> GLGQMLESMIDNTVRETVGAATSRDALPNTEASGPTHSKEIPALTAVETGATNPLVPSDTVQTRHVVQHRSRSESSIESFFARGACVTIMTVDNPASTTNKDKLFAVWKITYKDTVQLRRKLEFFTYSRFDMELTFVVTANFTETNNGHALNQVYQIMYVPPGAPVPEKWDDYTWQTSSNPSIFYTYGTAPARISVPYVGISNAYSHFYDGFSKVPLKDQSAALGDSLYGAASLNDFGILAVRVVNDHNPTKVTSKIRVYLKPKHIRVWCPRPPRAVAYYGPGVDYKDGTLTPLSTKDLTTY;> SPNIEACGYSDRVLQLTLGNSTITTQEAANSVVAYGRWPEYLRDSEANPVDQPTEPDVAACRFYTLDTVSWTKESRGWWWKLPDALRDMGLFGQNMYYHYLGRSGYTVHVQCNASKFHQGALGVFAVPEMCLAGDSNTTTMHTSYQNANPGEKGGTFTGTFTPDNNQTSPARRFCPVDYLLGNGTLLGNAFVFPHQIINLRTNNCATLVLPYVNSLSIDSMVKHNNWGIAILPLAPLNFASESSPEIPITLTIAPMCCEFNGLRNITLPRLQ;> GLPVMNTPGSNQYLTADNFQSPCALPEFDVTPPIDIPGEVKNMMELAEIDTMIPFDLSATKKNTMEMYRVRLSDKPHTDDPILCLSLSPASDPRLSHTMLGEILNYYTHWAGSLKFTFLFCGSMMATGKLLVSYAPPGADPPKKRKEAMLGTHVIWDIGLQSSCTMVVPWISNTTYRQTIDDSFTEGGYISVFYQTRIVVPLSTPREMDILGFVSACNDFSVRLLRDTTHIEQKALAQ;> XGAQVSSQKVGAHENSNRAYGGSTINYTTINYYRDSASNAASKQDFSQDPSKFTEPIKDVLIKTAPMLN;> MARAMAAAWPLLLVALLVLSWPPPGTGDVVVQAPTQVPGFLGDSVTLPCYLQVPNMEVTHVSQLTWARHGESGSMAVFHQTQGP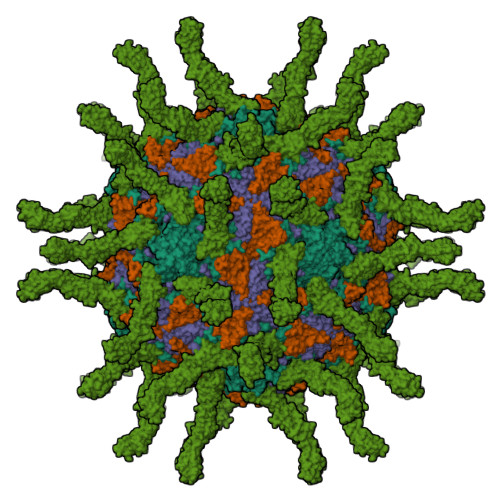SYSESKRLEFVAARLGAELRNASLRMFGLRVEDEGNYTCLFVTFPQGSRSVDIWLRVLAKPQNTAEVQKVQLTGEPVPMARCVSTGGRPPAQITWHSDLGGMPNTSQVPGFLSGTVTVTSLWILVPSSQVDGKNVTCKVEHESFEKPQLLTVNLTVYYPPEVSISGYDNNWYLGQNEATLTCDARSNPEPTGYNWSTTMGPLPPFAVAQGAQLLIRPVDKPINTTLICNVTNALGARQAELTVQVKEGPPSEHSGISRNAIIFLVLGILVFLILLGIGIYFYWSKCSREVLWHCHLCPSSTEHASASANGHVSYSAVSRENSSSQDPQTEGTRHHHHHH> MSRPRLNRLLVLEEAVRVADGAGGHRLDWQAKGEVWAEVTAGSGSERAGEFVTLASVPFTIVVRAAPVGAARRPRPEQRFREGARIF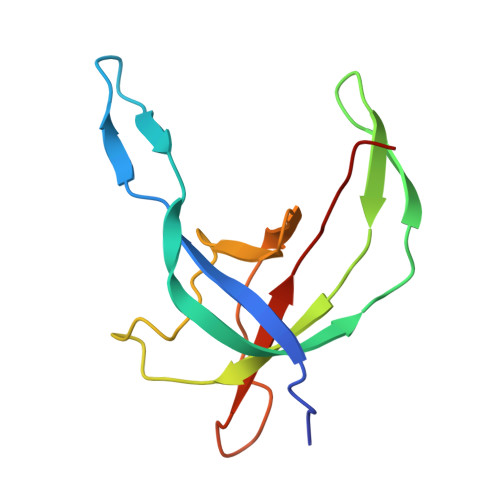RILAVAERDREGHYLSCFAREEVVA>MATKSVLMLGSGFVTRPTLDVLTDSGIKVTVACRTLESAKKLSAGVQHSTPISLDVNDDAALDAEVAKHDLVISLIPYTFHATVIKSAIRQKKHVVTTSYVSPAMMELDQAAKDAGITVMNEIGLDPGIDHLYAIKTIEEVHAAGGKIKTFLSYCGGLPAPESSDNPLGYKFSWSSRGVLLALRNAASFYKDGKVTNVAGPELMATAKPYFIYPGFAFVAYPNRDSTPYKERYQIPEADNIVRGTLRYQGFPQFIKVLVDIGFLSDEEQPFLKEAIPWKEATQKIVKASSASEQDIVSTIVSNATFESTEEQKRIVAGLKWLGIFSDKKITPRGNALDTLCATLEEKMQFEEGERDLVMLQHKFEIENKDGSRETRTSSLCEYGAPIGSGGYSAMAKLVGVPCAVAVKFVLDGTISDRGVLAPM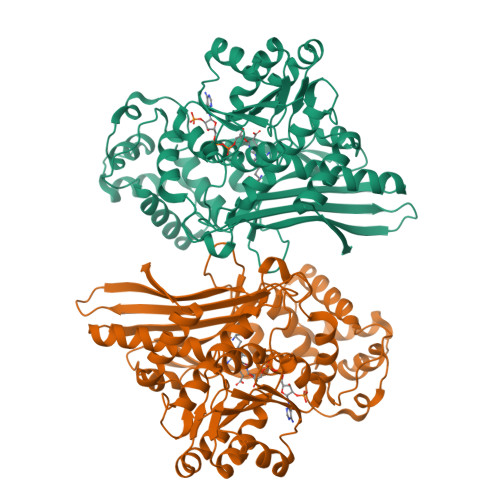NSKINDPLMKELKEKYGIECKEKVVA[8x]> SEACEMCRLGLPHGSFFELLRDWKKIEEFRNK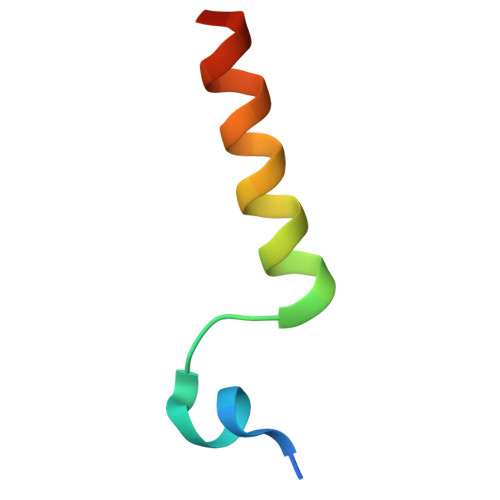S> ETLRGCPTHCHCEPDGRMLLRVDCSDLGLSELPSNL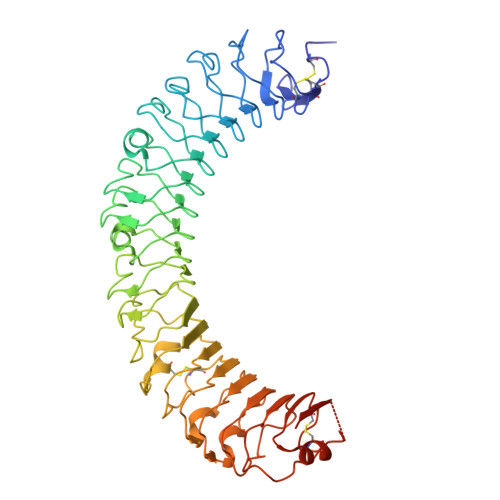SVFTSYLDLSMNNISQLLPNPLPSLRFLEELRLAGNALTYIPKGAFTGLYSLKVLMLQNNQLRHVPTEALQNLRSLQSLRLDANHISYVPPSCFSGLHSLRHLWLDDNALTEIPVQAFRSLSALQAMTLALNKIHHIPDYAFGNLSSLVVLHLHNNRIHSLGKKCFDGLHSLETLDLNYNNLDEFPTAIRTLSNLKELGFHSNNIRSIPEKAFVGNPSLITIHFYDNPIQFVGRSAFQHLPELRTLTLNGASQITEFPDLTGTANLESLTLTGAQISSLPQTVCNQLPNLQVLDLSYNLLEDLPSFSVCQKLQKIDLRHNEIYEIKVDTFQQLLSLRSLNLAWNKIAIIHPNAFSTLPSLIKLDLSSNLLSSFPITGLHGLTHLKLTGNHALQSLISSENFPELKVIEMPYAYQCCAFGVCENNGNNGDSVQCSPSGTHHHHHHHHHH> MKTITLYLDPASLPALNQLMDFTQNNEDKTHPRIFGLSRFKIPDNIITQYQNIHFVELKDNRPTEALFTILDQYPGNIELNIHLNIAHSVQLIRPILAYR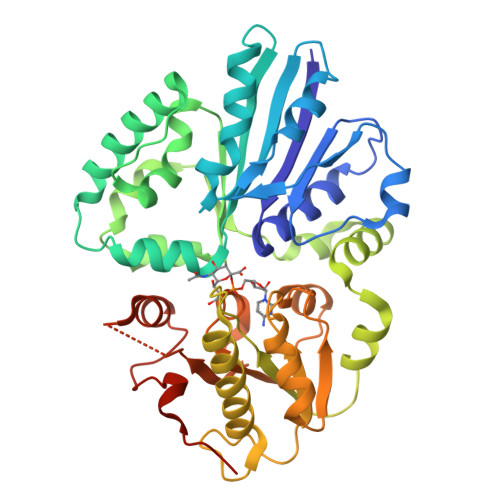FKHLDRVSIQQLNLYDDGSMEYVDLEKEENKDISAEIKQAEKQLSHYLLTGKIKFDNPTIARYVWQSAFPVKYHFLSTDYFEKAEFLQPLKEYLAENYQKMDWTAYQQLTPEQQAFYLTLVGFNDEVKQSLEVQQAKFIFTGTTTWEGNTDVREYYAQQQLNLLNHFTQAEGDLFIGDHYKIYFKGHPRGGEINDYILNNAKNITNIPANISFEVLMMTGLLPDKVGGVASSLYFSLPKEKISHIIFTSNKQVKSKEDALNNPYVKVMRRLGIIDESQVIFWDSLKQLGGGLEHHHHHH>UNNGAC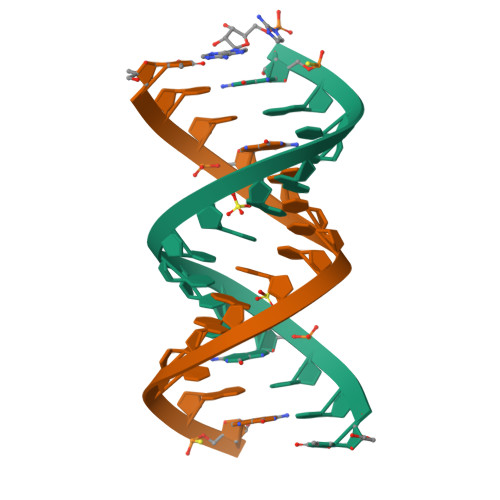UUAAGUCGG[2x]>[2x]MLLEAIFHEAKGSYAYPISETQLRVRLRAKKGDVVRCEVLYADRYASPEEELAHALAGKAGSDERFDYFEALLECSTKRVKYVFLLTGPQGEAVYFGETGFSAERSKAGVFQYAYIHRSEVFTTPEWAKEAVIYQIFPERFANGDPSNDPPGTEQWAKDARPRHDSFYGGDLKGVIDRLPYLEELGVTALYFTPIFASPSHHKYDTADYLAIDPQFGDLPTFRRLVDEAHRRGIKIILDAVFNHAGDQFFAFRDVLQKGEQSRYKDWFFIEDFPVSKTSRTNYETFAVQVPAMPKLRTENPEVKEYLFDVARFWMEQGIDGWRLDVANEVDHAFWREFRRLVKSLNPDALIVGEIWHDASGWLMGDQFDSVMNYLFRESVIRFFATGEIHAERFDAELTRARMLYPEQAAQGLWNLLDSHDTERFLTSCGGNEAKFRLAVLFQMTYLGTPLIYYG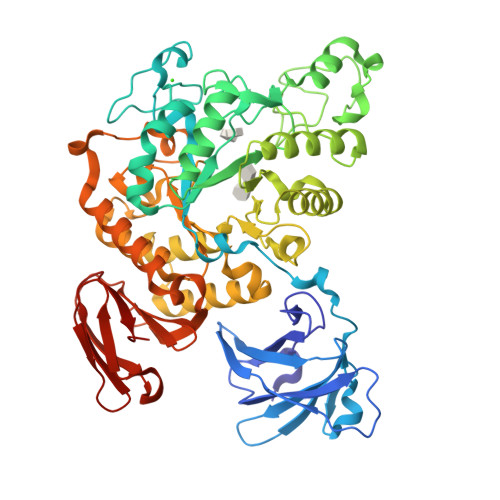DEIGMAGATDPDCRRPMIWEEKEQNRGLFEFYKELIRLRHRLASLTRGNVRSWHADKQANLYAFVRTVQDQHVGVVLNNRGEKQTVLLQVPESGGKTWLDCLTGEEVHGKQGQLKLTLRPYQGMILWNGR>MSLDKWEMERTDITMKHKLGGGQYGEVYEGVWKKYSLTVAVKTLKEDTMEVEEFLKEAAVMKEIKHPNLVQLLGVCTREPPFYIITEFMTYGNLLDYLRECNRQEVSAVVLLYMATQISSAMEYLEKKNFIHRDLAARNCLVGENHLVKVADFGLSRLMTGDTFTAHAGAKFPIKWTAPESLAYNKFSIKSDVWAFGVLLWEIATYG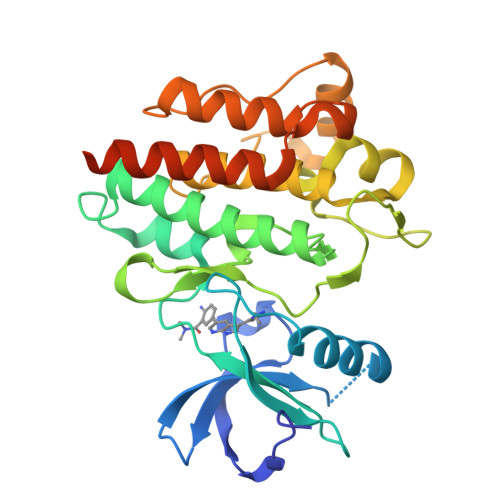MSPYPGIDPSQVYELLEKDYRMERPEGCPEKVYELMRACWQWNPSDRPSFAEIHQAFETMFQESSISDEVEKELGKRGEGHHHHHH[2x]> IRVNVLYSTPACYLWELNKANLSWSVKKDDFFPYADGPYMFWTGYFSSRPALKRYERLSYNFL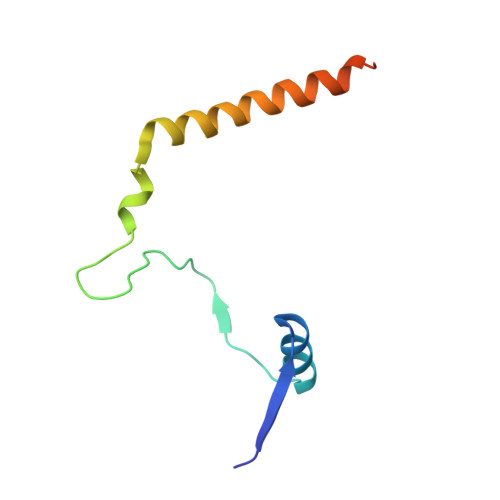QVCNQLEALAGPAANVGPYGS(2S,3R,11bR)-3-butyl-9,10-dimethoxy-1,3,4,6,7,11b-hexahydro-2H-pyrido[2,1-a]isoquinolin-2-amine | 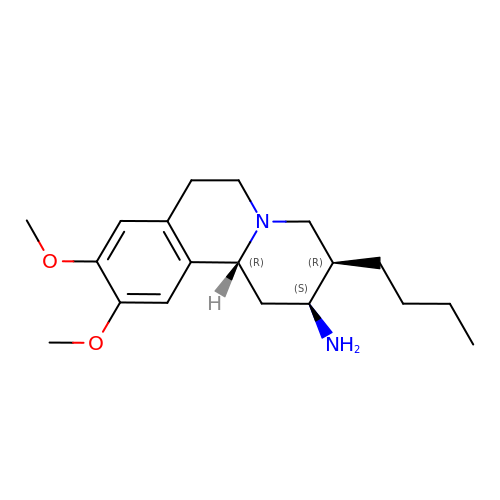C19 H30 N2 O2 | IYTDSNSLAQHLJL-HYVNUMGLSA-N>NSLPYGKINGTYKGTEKEKIKFSSEGSFDPDGKIVSYEWDFGDGNKSNEENPEHSYDKVGTYTVKLKVTDDKGESSVSTTTAEIKD[4x]

Clostridium histolyticum collagenases ColG and ColH are segmental enzymes that are thought to be activated by Ca2+-triggered domain reorientation to cause extensive tissue destruction. The collagenases consist of a collagenase module (s1), a variable number of polycystic kidney disease-like (PKD-like) domains (s2a and s2b in ColH and s2 in ColG) and a variable number of collagen-binding domains (s3 in ColH and s3a and s3b in ColG). The X-ray crystal structures of Ca2+-bound holo s2a (space group C2), Ca2+-free apo s2a (space group P61), Ca2+-bound holo s2b (space group P21) and two new forms of N-terminally truncated wild-type apo s2 (space groups P21 and P212121) are reported for the first time. Comparison of crystal structures of ColG s2 with crystal structures of ColH s2a and s2b suggests that despite common tertiary folds, PKD-like domains can be grouped into two subsets.

Similar to the molecules in the holo s2a crystal, the four apo s2a molecules are similar (average r.m.s.d. of 0.5 ± 0.2 Å), with molecules C and D being the most similar (r.m.s.d. = 0.2 Å) and molecules A and D being the most divergent (r.m.s.d. = 0.8 Å). Molecules A and B, as well as molecules C and D, are related by a noncrystallographic twofold. Temperature factors for each structure are relatively high, possibly as a consequence of the high solvent content in the crystal (61.8%). The holo and apo structures resemble each other (r.m.s.d. = 0.6 ± 0.2 Å). As expected, the most notable difference between the structures occurs near the N-terminus, where Ca2+ reorients the interacting residues Asn685 and Ser686. While neither structure could be refined using anisotropic B factors, comparison of B factors revealed that with the exception of the N-terminal residues, no significant change in B factors occurred upon Ca2+ binding. Unlike s2b or s2, s2a truncates β-strand A through an approximately 126° rotation of the ψ bond of Ile692. To accommodate the change, Tyr696 packs with Phe706 and is involved in a Δ4 Tyr corner, in which the side-chain hydroxyl group hydrogen-bonds to the backbone four residues prior to it. In the s2a structures the termini are the most flexible. As mentioned, the B-factor trends in all holo and apo s2a structures are similar despite the difference in crystal packing.> MAMHPRKDWYELTRATNWTPSYVTEEQLFPERMSGHMGIPLEKWESYDEPYKTSYPEYVSIQREKDAGAYSVKAALERAKIYENSD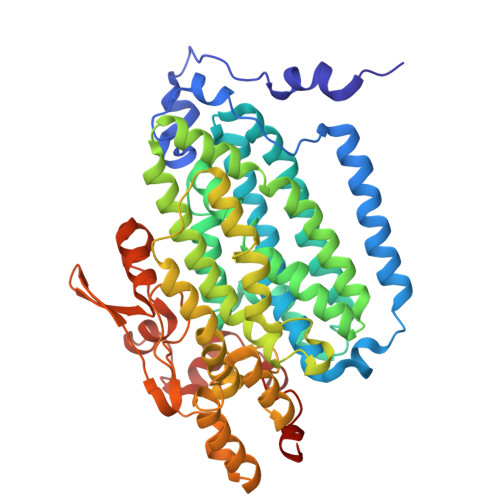PGWISTLKSHYGAIAVGEYAAVTGEGRMARFSKAPGNRNMATFGMMDELRHGQLQLFFPHEYCKKDRQFDWAWRAYHSNEWAAIAAKHFFDDIITGRDAISVAIMLTFSFETGFTNMQFLGLAADAAEAGDYTFANLISSIQTDESRHAQQGGPALQLLIENGKREEAQKKVDMAIWRAWRLFAVLTGPVMDYYTPLEDRSQSFKEFMYEWIIGQFERSLIDLGLDKPWYWDLFLKDIDELHHSYHMGVWYWRTTAWWNPAAGVTPEERDWLEEKYPGWNKRWGRCWDVITENVLNDRMDLVSPETLPSVCNMSQIPLVGVPGDDWNIEVFSLEHNGRLYHFGSEVDRWVFQQDPVQYQNHMNIVDRFLAGQIQPMTLEGALKYMGFQSIEEMGKDAHDFAWADKCK>MNENEPVSIWMHPEPAGRRSARSHRTLSRDQIVRAAVKVADTEGVEAASMRRVAAELGAGTMSLYYYVPTKEDLVELMVDEVIGETRLPDRPGPDWRAALTLAANEKRALWLRHPWLATAWRNGHPVWGPNSLRQQEFVLGTLGVFDLQVDELLSLIGLYNGYVESFVRNEVGWLEEARRTKVDMREWMRRSGPYAQQLVDSGEYPMFARVLAETVAPHMGPDQRFRSGLERLLDSIGASLDRLSPPGRSAAS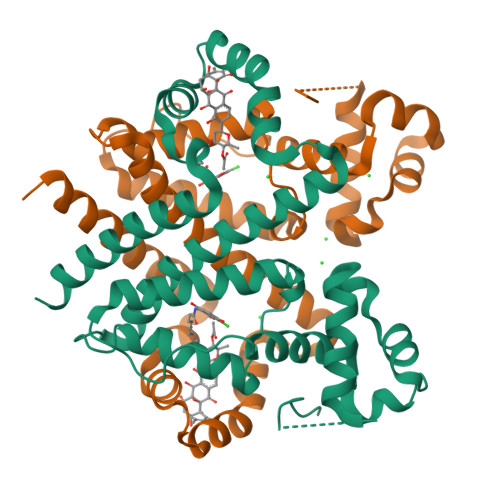ERPALALEHHHHHH[2x]2-AMINO-7,8-DIHYDRO-6-(1,2,3-TRIHYDROXYPROPYL)-4(1H)-PTERIDINONE | C9 H13 N5 O4 | 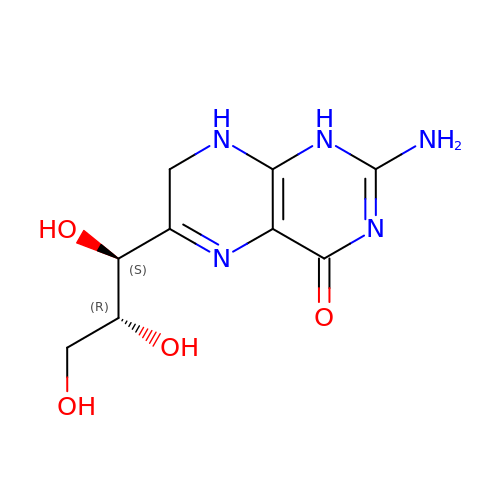YQIFAMYNGGOTFB-NJGYIYPDSA-N>GPTAAALERLTTEEVQGLSDVKTLVNQLYEALNVREHQLQKEVELTTQLETLQQELLPLEEKKLELEQVANRRSNWMAWAGLGLMSVQFGILARLTWWEYSWDIMEPVTYFVTYGTAMAAYAYFVLTREEYILNDVRDRQQLLLLHKKAKKTGFDVNQYNVLKDQIAKL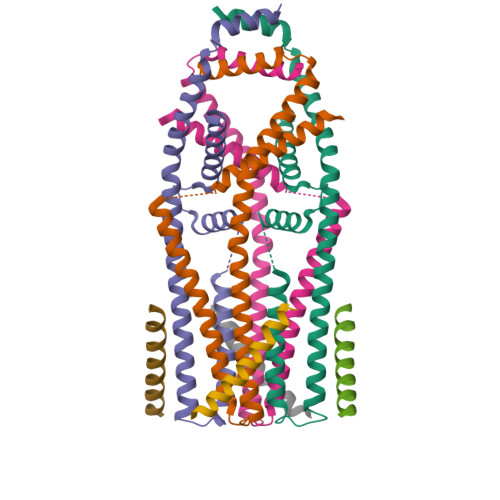ELDLKRLRDPLKLRLPPKAAASGSGSGENLYFQGSGGLLPEPHRTSFGIIRLILTVVPGLLIGAAISKNIANFL[8x]> TSFAE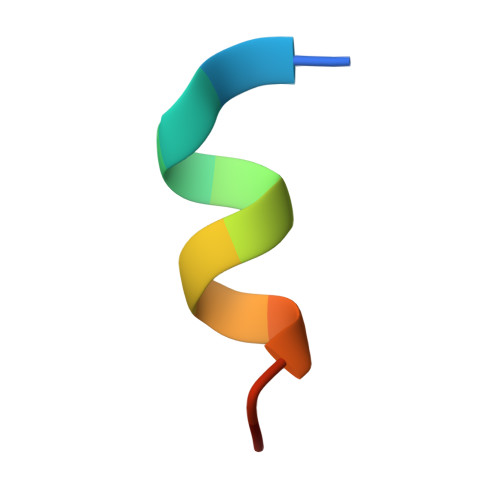YWALLSP> HHHHHHHTPSTQHSRPLTSEAFAALGAPALVYVRPIKAAEILADAPEGVEDLDLSPDQTLYAVCRADGERLAVLIDRDTAIAAALAH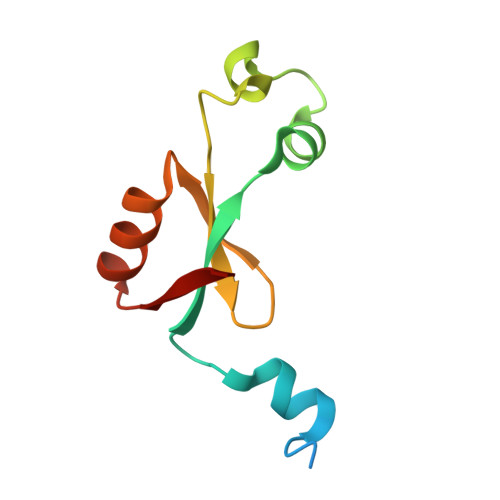ELAPVSVH>[2x]MASLPTANPDLVVSDAKKPKWSWRAIKSFAMGELEARKLKYPNTGTEALLMGILIEGTSFTSKFLRANKIMLYKVREETVKLLGKADMYFFSPEHPPLTEDAQRALDSALD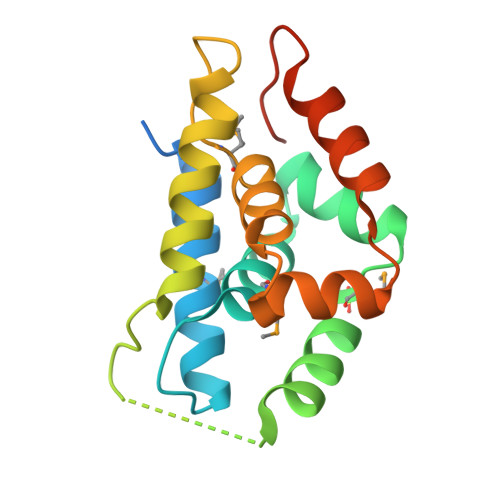QNLKAGGIGEVMPAHILLGIWSEVESPGHKILATLGFTDEKSKELESFASESGFLDELEHHHHHH>[4x]SELQTEGRTRNHGHNVCSTWGNFHYKTFDGDVFRFPGLCDYNFASDCRGSYKEFAVHLKRGPGQAEAPAGVESILLTIKDDTIYLTRHLAVLNGAVVSTPHYSPGLLIEKSDAYTKVYSRAGLTLMWNREDALMLELDTKFRNHTCGLCGDYNGLQSYSEFLSDGVLFSPLEFGNMQKINQPDVVCEDPEEEVAPASCSEHRAECERLLTAEAFADCQDLVPLEPYLRACQQDRCRCPGGDTCVCSTVAEFSRQCSHAGGRPGNWRTATLCPKTCPGNLVYLESGSPCMDTCSHLEVSSLCEEHRMDGCFCPEGTVYDDIGDSGCVPVSQCHCRLHGHLYTPGQEITNDCEQCVCNAGRWVCKDLPCPGTCALEGGSHITTFDGKTYTFHGDCYYVLAKGDHNDSYALLGELAPCGSTDKQTCLKTVVLLADKKKNVVVFKSDGSVLLNELQVNLPHVTASFSVFRPSSYHIMVSMAIGVRLQVQLAPVMQLFVTL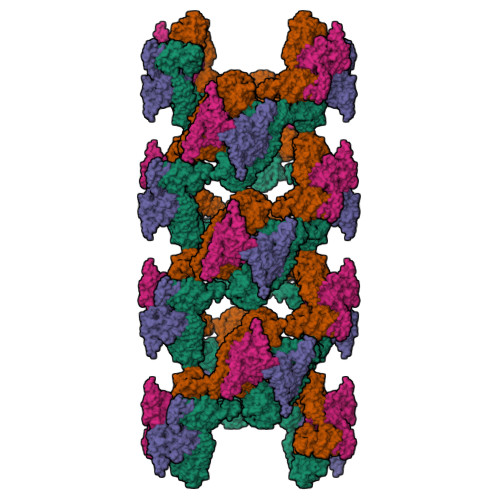DQASQGQVQGLCGNFNGLEGDDFKTASGLVEATGAGFANTWKAQSSCHDKLDWLDDPCSLNIESANYAEHWCSLLKKTETPFGRCHSAVDPAEYYKRCKYDTCNCQNNEDCLCAALSSYARACTAKGVMLWGWREHVCNKDVGSCPNSQVFLYNLTTCQQTCRSLSEADSHCLEGFAPVDGCGCPDHTFLDEKGRCVPLAKCSCYHRGLYLEAGDVVVRQEERCVCRDGRLHCRQIRLIGQSCTAPKIHMDCSNLTALATSKPRALSCQTLAAGYYHTECVSGCVCPDGLMDDGRGGCVVEKECPCVHNNDLYSSGAKIKVDCNTCTCKRGRWVCTQAVCHGTCSIYGSGHYITFDGKYYDFDGHCSYVAVQDYCGQNSSLGSFSIITENVPCGTTGVTCSKAIKIFMGRTELKLEDKHRVVIQRDEGHHVAYTTREVGQYLVVESSTGIIVIWDKRTTVFIKLAPSYKGTVCGLCGNFDHRSNNDFTTRDHMVVSSELDFGNSWKEAPTCPDVSTNPEPCSLNPHRRSWAEKQCSILKSSVFSICHSKVDPKPFYEACVHDSCSCDTGGDCECFCSAVASYAQECTKEGACVFWRTPDLCPIFCDYYNPPHECEWHYEPCGNRSFETCRTINGIHSNISVSYLEGCYPRCPKDRPIYEEDLKKCVTADKCGCYVEDTHYPPGASVPTEETCKSCVCTNSSQVVCRPEEGKILNQTQDGAFCYWEICGPNGTVEKHFNICSITHHHHHH> MAYFLDFDERALKEWRKLGSTVREQLKKKLVEVLESPRIEANKLRGMPDCYKIKLRSSGYRLVYQVID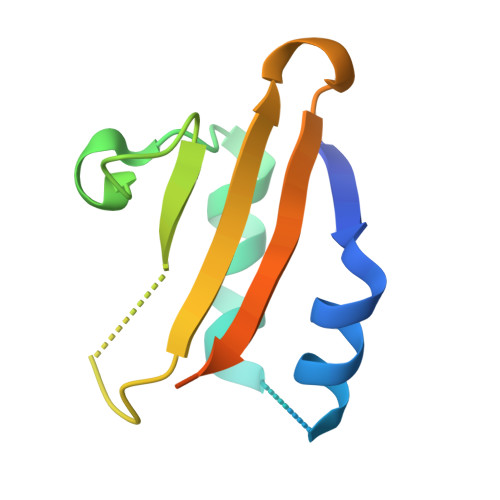EKVVVFVISVGKAERSEVYSEAVKRIL> HLSDMLQQLHSVNASKPSERGLVRQEEAEDPACIPIFWVSKWVDYSDKYGLGYQLCDNSVGVLFNDS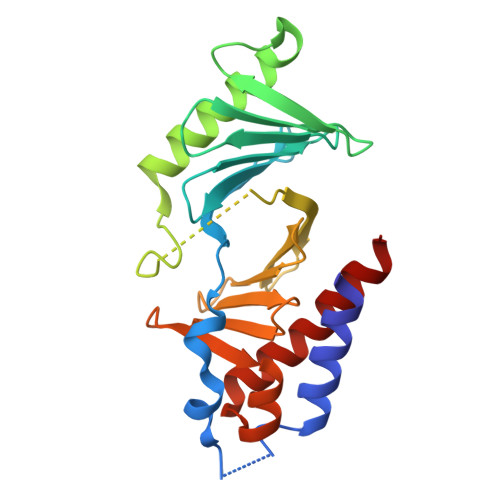TRLILYNDGDSLQYIERDGTESYLTVSSHPNSLMKKITLLKYFRNYMSEHLLKAGANITPREGDELARLPYLRTWFRTRSAIILHLSNGSVQINFFQDHTKLILCPLMAAVTYIDEKRDFRTYRLSLLEEYGCCKELASRLRYARTMVDKLLSSR>[2x]GSDDLVGVSVRPKVPLRTMSYKLAIDMSHFIKEKGGLE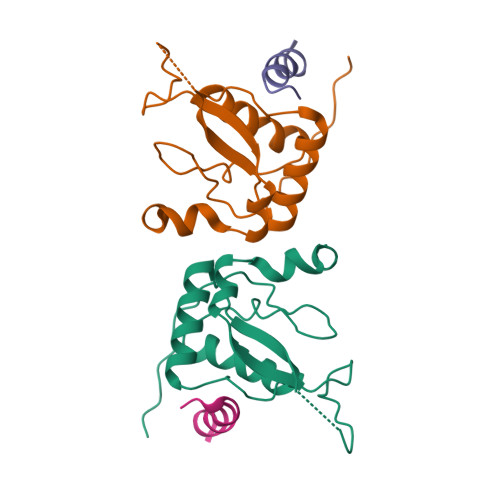GIYYSARRHRILDIYLEKEEGIIPDWQDYTSGPGIRYPKTFGWLWKLVPVNVSDEAQEDEEHYLMHPAQTSQWDDPWGEVLAWKFDPTLAYTYEAYVRYPEEFGS;>AYQQGQNQLYNELNLGRR[2x]> 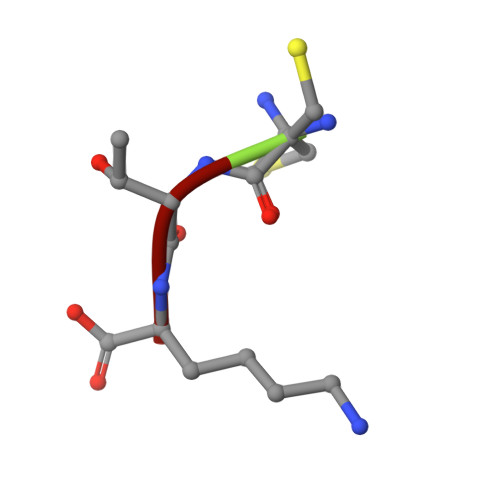CTK Purine nucleoside phosphorylase (PNP) is central to purine salvage mechanisms in Plasmodium parasites, the causative agents of malaria. Purine nucleoside phosphorylase (PNP) in Plasmodium forms a key enzyme in the recycling of predominantly host-derived purines, catalysing the phosphorolysis of inosine to produce the major purine precursor for the salvage pathway, hypoxanthine, and ribose-1-phosphate. Crystal structures and sequence homology studies have distinguished two broad families of PNP enzymes: those that form trimers (such as the mammalian PNPs, Type 2) and those that are hexameric (such as E.coli PNP (EcPNP), Type 1). Crystallographic studies of PfPNP have shown it forms a hexameric assembly suggesting its closer alignment with the Type 1 PNP group, although functionally it has been noted that, unlike other hexameric PNPs, adenosine is not a substrate for PfPNP.

The asymmetric unit consists of one hexamer of PfPNP in which there are six very similar, but not identical, subunits. In accordance with the shapes, sizes and positions of electron density observed within the active site, the products hypoxanthine base, ribose sugar and arsenate anion (AsO4) – formed from the irreversible arsenolysis of inosine followed by hydrolysis of the ribose-1-arsenate – were modelled in to the observed electron density map. In all subunits, the arsenate moiety is stabilised mainly by two arginine side chains (Arg 88 and Arg 45' of the neighbouring subunit) and further hydrogen bonds are formed with donors from the hydroxyl group of Ser 91 and the backbone amino groups of Gly 23 and Ser 91. However the participation of the Arg 27 residue in the anion binding pocket, where its guanidinium side chain forms charged hydrogen bonds with the arsenate molecule, has not been observed in structures with sulphate bound. In the PfPNP-HRA complex, in five of the subunits the Arg 27 side chain points toward the active site ('closed' conformation, average torsion angle χ1 = 163° and χ2 = 175°) and forms hydrogen bonds with oxygen atoms of the arsenate ion. By contrast, in chain F this arginine is in an 'open' conformation with its side chain pointing away from the active site (torsion angle χ1 = 178° and χ2 = 75°) and hence does not interact with the arsenate ion. Similar to the PfPNP-Imm complex, the carboxylate group of the Asp 206 side chain interacts directly with N7 of the hypoxanthine, and has been proposed to be the general acid/base for protonation of N7 of the substrate in the transition state. In the PfPNP-HRA complex, although all active sites are occupied, in four subunits (A,B,D,E) the active site loop is ordered – indicative of a catalytically-active form – whereas its disorder in subunits C and F may reflect the start of a transition in which the enzyme adopts a 'relaxed state' to release the products of arsenolysis. At this point the C1' atom lies equidistant between the N9 of the base and the incoming phosphate/arsenate oxygen nucleophile.

>[6x]MDNLLRHLKISKEQITPVVLVVGDPGRVDKIKVVCDSYVDLAYNREYKSVECHYKGQKFLCVSHGVGSAGCAVCFEELCQNGAKVIIRAGSCGSLQPDLIKRGDICICNAAVREDRVSHLLIHGDFPAVGDFDVYDTLNKCAQELNVPVFNGISVSSDMYYPNKIIPSRLEDYSKANAAVVEMELATLMVIGTLRKVKTGGILIVDGCPFKWDEGDFDNNLVPHQLENMIKIALGACAKLATKYALEHHHHHH>[6x]GQEEGEDNGGEDNKKLRGALSSAILSEKPNVKWEDVAGLEGAKEALKEAVILPVKFPHLFKGNRKPTSGILLYGPPGTGKSYLAKAVATEANSTFFSVSSSDLVSKWMGESEKLVKQLFAMARENKPSIIFIDEVDALTGTRGEGESEASRRIKTELLVQMNGVGNDSQGVLVLGATNIPWQLDSAIRRRFERRIYIPLPDLAARTTMFEINVGDTPCVLTKEDYRTLGAMTEGYSGSDIAVVVKDALMQPIRKIQSATHFKDVSTEDDETRKLTPC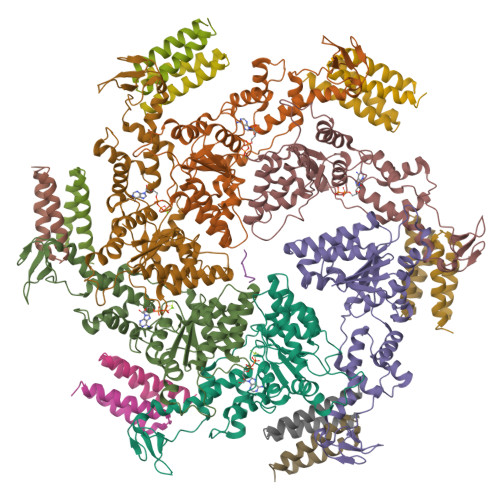SPGDDGAIEMSWTDIEADELKEPDLTIKDFLKAIKSTRPTVNEDDLLKQEQFTRDFGQEGNGGGGSGGGGSGGGGSGGGMAVDMFIKIGDVKGESKDKTHAEEIDVLAWSWGMSQSGSMHMGGGGGAGKVNVQDLSFTKYIDKSTPNLMMACSSGKHYPQAKLTIRKAGGENQVEYLIITLKEVLVSSVSTGGSGGEDRLTENVTLNFAQVQVDYQPQKADGAKDGGPVKYGWNIRQNVQAG;> XDEIVNKVLX;>[12x]MASNAARVVATAKDFDKVGLGIIGYYLQLYAVELILSEEDRSQEMTALATELLDTIEAFKKEIGGESEAEDSDKSLHVMNTLIHDQEKAKIYMLNFTMSLYNEKLKQLKDGPWDVMLKRSLWCCIDLFSCILHLWKENISETSTNSLQKRIKYCKIYLSKLAKGEIGSSDEKTLDYADFADDSEEIKDEDVDHQTSDLENNNNDKVEGLAPKDQTTSYEPVDEVPEFIDDADSVNEEEQTVDKNEDAITKDEQQVVKKEVDLTRPSAPSEPAAAEHKSYTKDELTKIMDRASKIEQIQKLAKYAISALNYEDLPTAKDELTKALDLLNSI The retinoblastoma tumor suppressor (Rb) is a multifunctional protein that primarily regulates the cell cycle but also has roles in cellular differentiation, DNA damage response, and apoptosis. Essential functions of Rb occur through its pocket domain, which is necessary for regulating binding interactions with E2F transcription factors and transcription repressors that bind via an LxCxE motif. The pocket domain is the most highly conserved region of the multidomain protein, as well as the most frequent site of mutations. Protein X-ray crystallography of four missense variants reveals how mutations destabilize the protein fold and inhibit E2FTD or LxCxE binding.

At 25 °C, the majority of variants that strongly reduce E2F1TD binding (by 10-fold or greater) are located at the E2FTD-binding cleft; these include S534R (820-fold), K530I (63-fold); E533K (59-fold); E544K (34-fold); R656Q (13-fold); H555Y (12-fold); and K548N (10-fold). Within the cyclin fold of subdomain A, the greatest destabilizing effects (ΔTm) are caused by E554K (−7.0 ± 0.5 °C), E533K (−6.4 ± 0.5 °C), E492Q (−5.4 ± 0.8 °C), A490V (−5.1 ± 0.6 °C), K462E (−5.0 ± 0.5 °C), E539D (−4.9 ± 0.5 °C), A490T (−4.7 ± 1.0 °C), and A488V (−4.1 ± 0.6 °C). For E554K and E533K, we sought to understand the structural basis for large reductions in RbP-E2F1TD binding as well as substantial decreases in thermostability. Remarkably, the crystal structure of E533K shows something similar in which the mutated lysine sidechain creates a salt bridge triad with E554 and E551 in a manner that occludes the Y411(E2F1TD)-binding pocket. Together, the variant structures of E533K and E554K reveal a structural basis for the disruption of E2FTD binding. However, from these structures alone, it is not clear how the mutations induce fold destabilization. In the structures of RbP-E2F2TD RbP-E2F1TD, both E554 and E533 form A/B subdomain-spanning salt bridges to K653. It is possible that the loss of the salt bridge interactions contributes to the large destabilization effects observed for these variants.

>GEFNTIQQLMMILNSASDQPSENLISYFNNCTVNPKESILKRVKDIGYIFKEKFAKAVGQGCVEIGSQRYKLGVRLYYRVMESMLKSEEERLSIQNFSKLLNDNIFHMSLLACALEVVMATYSRSTSQNLDSGTDLSFPWILNVLNLKAFDFYKVIKSFIKAEGNLTREMIKHLERCEHRIMESLAWLSDSPLFDLIKQSKDREGPTDHLESACPLNLPLQNNHTAADMYLEPVRAPKKKSTSLSLFYKKVYRLAYLRLNTLCERLLSEHPELEHIIWTLFQHTLQNEYELMRDRHLDQIMMCSMYGICKVKNIDLKFKIIVTAYKDLPHAVQETFKRVLIKEEEYDSIIVFYNSVFMQRLKTNILQYASTRPPTLAPIPHIPFMQRLKT[2x]>[2x]IKDPQTGAPVPLRALINNVSGYVIKTEMYTEVKNAKGEWVFKSLGKPGSMHLRPIATPYPVKEWLQPKRYKAHLMGTTYVYDFPELFRQASSSQWKNFSADVKLTDDFFISNELIEDENGELTEVEREPGANAIGMVAFKITVKTPEYPRGRQFVVVANDITFKIGSFGPQEDEFFNKVTEYARKRGIPRIYLAANSGARIGMAEEIVPLFQVAWNDAANPDKGFQYLYLTSEGMETLKKFDKENSVLTERTVINGEERFVIKTIIGSEDGLGVECLRGSGLIAGATSRAYHDIFTITLVTCRSVGIGAYLVRLGQRAIQVEGQPIILTGAPAINKMLGREVYTSNLQLGGTQIMYNNGVSHLTAVDDLAGVEKIVEWMSYVPAKRNMPVPILETKDTWDRPVDFTPTNDETY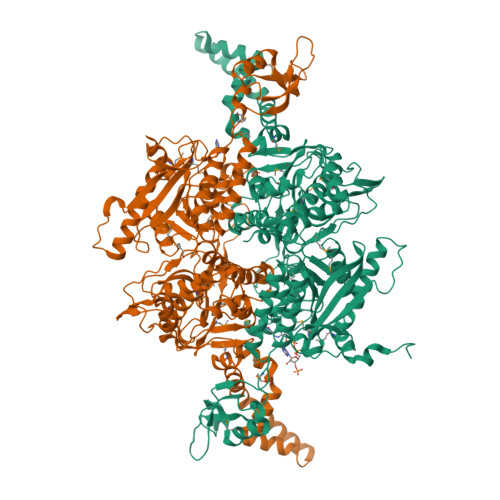DVRWMIEGRETESGFEYGLFDKGSFFETLSGWAKGVVVGRARLGGIPLGVIGVETRTVENLIPADPANPNSAETLIQEPGQVWHPNSAFKTAQAINDFNNGEQLPMMILANWRGFSGGQRDMFNEVLKYGSFIVDALVDYKQPIIIYIPPTGELRGGSWVVVDPTINADQMEMYADVNARAGVLEPQGMVGIKFRREKLLDTMNRLDDKYRELRSQLSNKSLAPEVHQQISKQLADRERELLPIYGQISLQFADLHDRSSRMVAKGVISKELEWTEARRFFFWRLRRRLNEEYLIKRLSHQVGEASRLEKIARIRSWYPASVDHEDDRQVATWIEENYKTLDDKLKGLKLESFAQDLAKKIRSDHDNAIDGLSEVIKMLSTDDKEKLLKTLK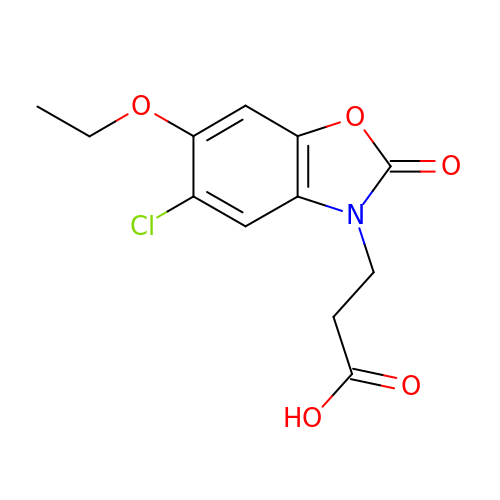3-(5-chloranyl-6-ethoxy-2-oxidanylidene-1,3-benzoxazol-3-yl)propanoic acid | C12 H12 Cl N O5 | KPOKXAQERBEAHE-UHFFFAOYSA-N>MAHHHHHHMSRLIVVSNRVAIGEDTRPSAGGLAVGVMDALQETGGVWFGWNGEIVGTPDAAPAIRRDGNVTYATVGLTRRDYDQYYRGFSNATLWPVFHYRGDLARFDRQEYAGYLRVNAMLAKQLAALLRPDDLIWVHDYHLLPFAHALRELGVKNPIGFFLHIPFPSPDVLRLVPPHDELVKFMCAYDVTGFQTDADRQAFTDYIERRGIGTASEDGMLHAHGRVVKVAAYPIGVYPDAIAQAAVQYGARKPVK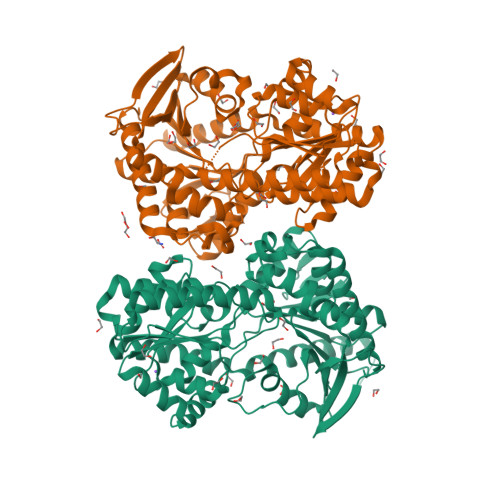MLRDALGGRKLVMSVDRLDYSKGLVERFQAFERMLANAPGWQGRVSLVQIAPPTRSDVQTYQRIRETLEGEAGRINGRFSQLDWTPIQYLNRKYERNLLMAFFRMSQVGYVTPLRDGMNLVAKEYVASQDPADPGVLVLSEFAGAAAELTGALLVNPYDLSQMADALERALSMPLAERQARHEENLARLRANDLSVWRDTFVADLRSVAAAASVTQRAGRRIAHA[2x]> GSHMASSDDVTVVYQNGLPVISVRLPSRRERCQFTLKPISDSVGVFLRQLQEEDRGIDRVAIYSPDGVRVAASTGIDLLLLDDFKLVINDLTYHVRPPKRDLLSHENAATLNDVKTLVQQLYTT

The mitochondrial Ca2+ uniporter complex (mtCU) formed across the IMM is the predominant channel responsible for mediating Ca2+ uptake into the matrix. The principal components of mtCU are the pore-forming, mitochondrial Ca2+ uniporter (MCU) subunits that oligomerize into tetrameric channels. The conserved Asp-Ile-Met-Glu (DIME) motif in each subunit forms the Ca2+ selectivity filter at the intermembrane space (IMS)-exposed channel entrance by symmetric arrangement of the four subunits. Indeed, we and others demonstrated that binding of Ca2+ or Mg2+ to an MCU regulating acidic patch (MRAP) on the NTD destabilizes domain self-association and inhibits mtCU activity.

Here, we re-crystallized the human MCU-NTD in the absence of divalent cations, determining a structure to 1.6 Å resolution; moreover, this structure is the highest-resolution WT MCU-NTD structure we have achieved to date in the absence of divalent cations, providing the best starting point to investigate the effects of Ca2+ and Mg2+ binding on conformation and dynamics using in silico simulations. Given the high sequence similarity to MCUb-NTD and since no high-resolution structure exists for MCUb, this new structure is also the best template to homology model MCUb-NTD. Similar to our previous crystal structures, the present WT MCU-NTD shows a β-grasp-like fold, consisting of two helices, held between two β-sheets. The C-terminus (i.e. residues 166–189) is not resolved, suggesting the region is dynamic under our crystallization conditions. The central α1-helix (residues 108–118) is approximately perpendicular to the second capping α2-helix (residues 141–146). The antiparallel β1, β2 and β3 strands of the first β-sheet are made up of residues 76–80, 83–88 and 97–100, respectively, while the antiparallel β4, β5 and β6 strands consist of residues 125–128, 149–153 and 156–160, respectively. Notably, the residues that make up MRAP in human MCU-NTD (i.e. D131, D147, D148) are not fully conserved in human MCUb-NTD at the primary (i.e. D116, N132, D133) and three-dimensional (3D) structural levels. Over the 1 μs simulation time, this single Ca2+ ion underwent 95,239 total interactions with MCU-NTDWT, with ∼97 % contacts occurring with MRAP residues D131, D147 and D148 (i.e. 29,851, 29,594 and 32,478 interactions, respectively). Collectively, these MCU-NTDWT MD data suggest that single Ca2+ binding occurs preferentially in MRAP, increasing L5 rigidity, while additional Ca2+ ions interact with the central helix, destabilizing the structure. Collectively, the data suggest that an ∼10 °C increase in temperature favours MCU-NTD structural stability and decreased dynamics in contrast to MCUb-NTD, which is destabilized by the higher temperature.>[4x]MAEAASCARKGTKYAEGTQPFTVLIEGNIGSGKTTYLNHFEKYKNDICLLTEPVEKWRNVNGVNLLELMYKDPKKWAMPFQSYVTLTMLQSHTAPTNKKLKIMERSI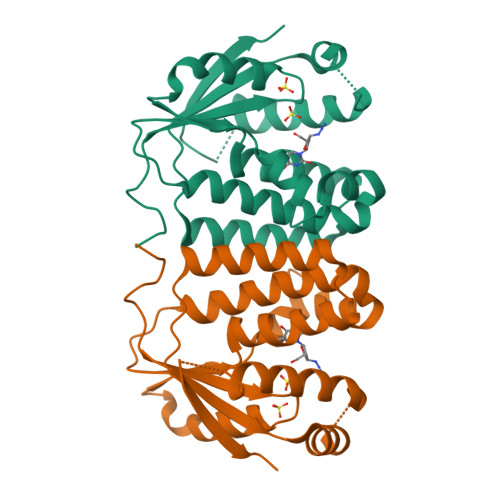FSARYCFVENMRRNGSLEQGMYNTLEEWYKFIEESIHVQADLIIYLRTSPEVAYERIRQRARSEESCVPLKYLQELHELHEDWLIHQRRPQSCKVLVLDADLNLENIGTEYQRSESSIFDAIS Single-stranded RNA bacteriophages (ssRNA phages) are positive-sense RNA viruses that have shown specificity for gram-negative bacteria by exploiting host retractile pili, including T4P6. Acinetobacters have type IV pili (T4P), which are involved in twitching motility, surface adhesion, biofilm formation, and natural transformation in gram-negative bacteria. Our study delves into the interaction between Acinetobacter phage AP205 and type IV pili. Using cryo-electron microscopy, we solve structures of the AP205 virion with an asymmetric dimer of maturation proteins, the native Acinetobacter type IV pili bearing a distinct post-translational pilin cleavage, and the pili-bound AP205 showing its maturation proteins adapted to pilin modifications, allowing each phage to bind to one or two pili.

To investigate the recognition mechanism between AP205 and T4P, we employed single-particle cryo-EM to obtain a structure of the AP205/T4P complex. The two copies of Mat exhibit different conformations: One Mat (referred as outer Mat) extends further to elevate its apical domain away from the capsid shell while the other Mat (referred as inner Mat) is embedded deeper within the capsid and has a larger bending angle between the central and basal domains. Within the T4P-Mat complex, the apical domain of each Mat specifically plugs into the groove formed by three adjacent pilin subunits within the T4P (referred to as Pilins 1, 2). Notably, the C-terminal Ser147 of Pilins 1 and 2 are positioned near β3 and β7 of the Mat apical domain, respectively. Apparently, glycosylation at these two serines can prevent binding of AP205 Mat. It is likely that the substoichiometric glycosylation of pilins allows AP205 to bind to unglycosylated sites on the T4P. We also observed that the internal cleavage site of Pilin 3 at Ser79 is located at the binding interface for the apical domain. This cleavage allows Ser79 to move ~13 Å away from Gly78, allowing its interaction with β8 of the Mat. In the natural environment, during the interaction of AP205 with A.gp16, it is plausible that multiple T4P from the same cell come into close proximity. This allows the pair of Mat proteins from a single phage to simultaneously bind to two pili, as shown in the major class of our single-particle cryo-EM structure of the in-vitro reconstituted AP205-pili complex.

>[18x]TLIELMIVVAIIGILAAIAIPQYQNYIAKSQVSRVMSETGSLKTVIETCILDGKTAANCELGWTNSNLLG;>STAAVTGQTGLTITYPASATESAAIQGTFGNSAAIKIKNQTLTWTRTPEGAWSCATTVEAKFKPAGCAS[18x];> MNMYKWVPESIRDSGEGQPSYSNNGDYAPSGPWVAAGIHTMPQSLRDSMRNSIMVTAQARRDVIGPEWGPDGRFTGYASVIGTPDPKPADIVNKFTVERRPVSNGNFQQRVKAGDIVVAPYTSDGKITVKLVAGQKDISSTPDYDYRIDSSLASSAGFVVAGERWYYTKRHFIIPRYFQNWRMRRRKYVTGWVMPTFYSPKEIFNRLKDSLVPDTGLVTQVWADNNTKRMDFLTAMAEIPQTLSSFLDALGYLGSLIKDFKRRRFFLNKAHQRIRNKLGVSFAERRSQIVSKYDRKIASARKPAIIVKLRQRKEKALKALDKMRVREEKKMIREFATQAASLWLSFRYEIMPLYYQSQDVLDVIANSTSEFMTSRDFVAKAINIGIPLEWNLDQENLVSQPRHNVMVKSKLSPENNIGKTLSVNPFTTAWELLTLSFVVDWFVNFGDVIAGFTGGYSDDSGATASWRFDDKKVFHLKNIPSAMVIVDINFYTRQVIDPRLCGGLAFSPKLNLFRYLDAMSLSWNRSRLKISRAT> KEVWQVILKPKGLGQTKNLIGIYRLCLTSKTISFVKLNSEAAAVVLQLMNIRRCGHSENFFFIEVGRSAVTGPG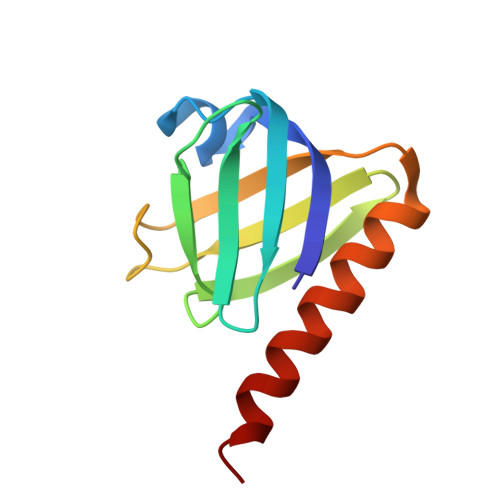EFWMQVDDSVVAQNMHETILEAMRAMSDAFR>TAPAAASRASRVPLSGMALPVVSAKTVQLNDGGLVRTVHLPAPNVAGLLSAAGVPLLQSDHVVPAATAPIVEGMQIQVTRNRIKKVTERLPLPPNARRVEDPEMNMSREVVEDPGVPGTQDVTFAVAEVNGVETGRLPVANVVVTPAHEAVVRVGTKPGTEVPPVIDGSIWDAIAGCEAGGNWAINTGNGYYGGVQFDQGTWEANGGLRYAPRADLATREEQIAVAEVTRLRQGWGAWPVCAARAGAR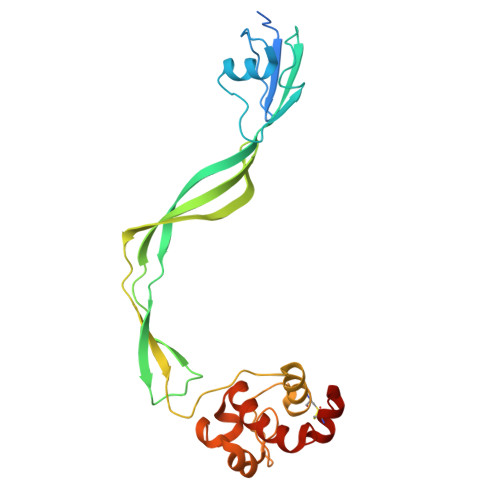[2x]>[2x]GSKKRQRFVDKNGRCNVQHGNLGSETSRYLSDLFTTLVDLKWRWFFVSLAVLFLLLNTAFATLYMLGSAPIANQFPAGFGGAFFFSVETLATVGYGDMHPQTVYAHWIATLEIFVGMSSIALATGCAFIKMSQPKKRAETLMFSEHAVISMRDGKLTLMFRVGNLRNSHMVSAQIRCKLLKSRQTPEGEFLPLDQLELDVGFSTGADQLFLV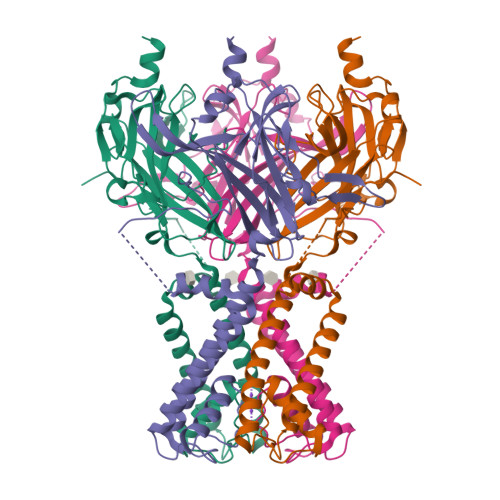SPLTICHVIDAKSPFYDLSQRSMQTEQFEVVVILEGIVETTGMTCQARTSYTEDEVLWGHRFFPVISLEEGFFKVDYSQFHATFEVPTPPYSVKEQEEMLLMSSPLVPR Collagens are an essential component of the extracellular matrix (ECM) of all higher organisms. All of them share as defining feature the so-called collagen triple helix; a structural element that is formed by three individual polypeptide chains (reviewed in1–3). The three-dimensional structure of this extended, non-globular domain requires a glycine in every third position, leading to a repetition of the triplet motif Gly-Xaa-Yaa. One of the important interaction partners of collagens in cartilage is the cartilage oligomeric matrix protein (COMP) a member of the thrombospondin family of proteins, also referred to as TSP-5.

To elucidate possible binding interfaces we used an unpublished crystal structure of a collagen peptide with the sequence Ac-(POG)4LKGHRGFTGLQG-(POG)4-NH2, which resembles the C-terminal COMP binding motif of collagen II. Docking was performed with ClusPro and the best 10 models analysed by manual inspection. Furthermore, no metal ion would be necessary for this interaction. In the docked model, Asp593 of COMP form hydrogen bonds to the arginine and lysine of the middle strand (Fig. 8 dark blue) and the histidine of the middle chain (Fig. 8 light blue). Asp594 and Asp595 interact with the lysine of the middle strand. To test this model, we mutated all three aspartates to alanine residues and expressed and purified the protein. To our surprise the mutant behaved similar to the wildtype in binding assays, falsifying the proposed model. By testing a generated triple mutant replacing all three aspartate residues by alanines, we could show that this potential MIDAS motif is not involved in the binding of COMP to collagen. Close to the C-terminal propeptide, the sequence 1128GLKGHR1133 matches this consensus. Interestingly, this motif (GXKGHR) overlaps with the recognition sequence of various other collagen binders (heparin, PEDF).

>XPPGPPGPPGPPGLKGHRGFTGLQGPPGPPGPPGPPGX[3x]> EKFGK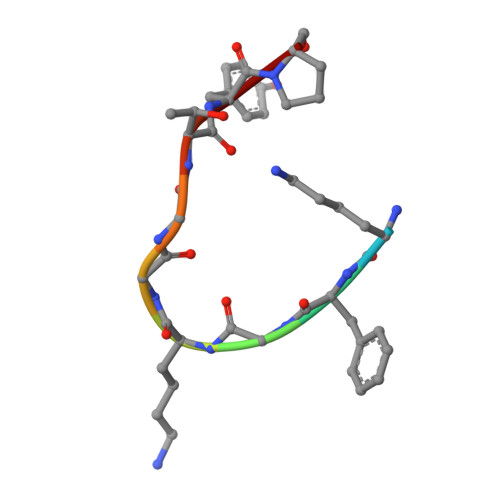GGTYP> MRVLLIHSDYIEYEVKDKALKNPEPISEDMKRGRMEEVLVAFISVEKVDEKNPEEVSLKAIEEISKVAEQVKAENVFVYPFAHLSSELAKPSVA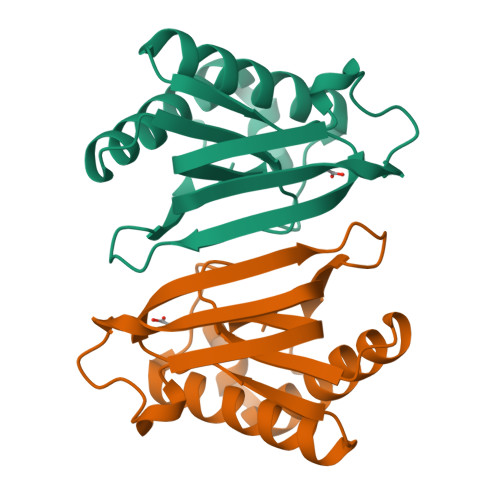MDILNRVYQGLKERGFNVGKAPFGYYKAFKISCKGHPLAELSRTIVPEE> EGKITPVSVKKVDDKVTLYKTTATADSDKFKISQILTFNFIKDKSYDKDTLVLKATGNINSGFVKPNPNDYDFSKLYWGAKYNVSISSQSNDSVNVVDYAPKNQNEEFQVQNTLGYTFGGDISISNGLSGGLNGNTAFSETINYKQESYRTTLSRNTNYKNVGWGVEAHKIMNNGWGPYGRDSFHPTYGNELFLAGRQSSAYAGQNFIAQHQMPLLSRSNFNPEFLSVLSHRQDGAKKSKITVTYQREMDLYQIRWNGFYWAGAN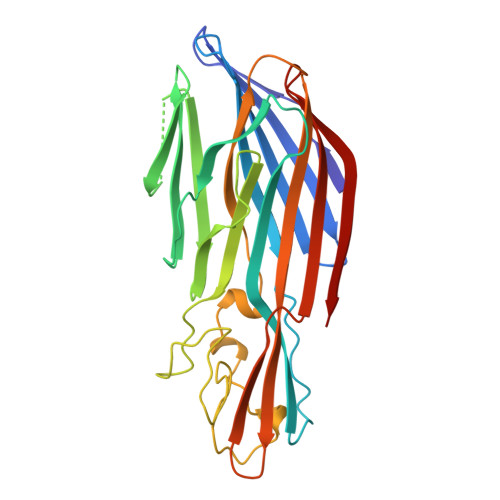YKNFKTRTFKSTYEIDWENHKVKLLDTKETENNK> GSMSGKASTEGSVTTEFLSDIIGKTVNVKLASGLLYSGRLESIDGFMNVALSSATEHYESNNNKLLNKFNSDV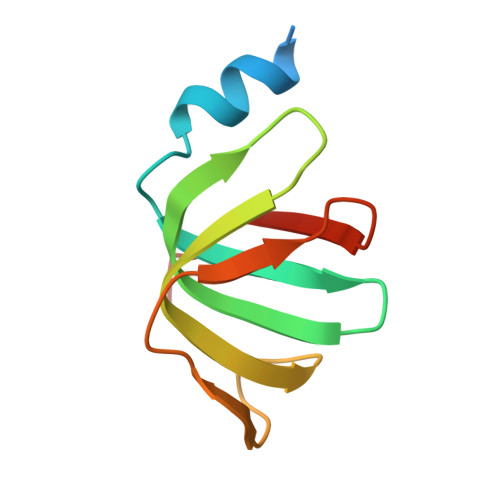FLRGTQVMYISEQKI>[4x]GPLGSSKTKPFTLPILTISEMSNSRFPVPIDSLHTSPTENIVVQCQNGRVTLDGELMGTTQLLPSQICAFRGTLTRSTSRASDQADTPTPRLFNYYWHIQLDNLNGTPYDPAEDIPAPLGTPDFRGKVFGVASQRNPDSTTRAHEAKVDTTSGRFTPKLGSLEITTESDDFDPNQPTKFTPVGVGVDNEAEFQQWSLPNYSGQFTHNMNLAPAVAPNFPGEQLLFFRSQLPSSGGRSNGVLDCLVPQEWVQHFYQESAPAQTQVALVRYVNPDTGRVLFEAKLHKLGFMTIAKNGDSPITVPPNGYFRFESWVNPFYTLAPMGTGNG

NoVs recognize specific glycan ligands as host attachment factors or receptors for infection. NoVs interact with HBGAs or other glycans through their capsid protrusions that are built by the dimeric protruding (P) domain of NoV capsid protein (VP1). Genogroup II (GII) noroviruses consist of human noroviruses (huNoVs) that generally bind histo-blood group antigens (HBGAs) as host factors and three porcine norovirus (porNoV) genotypes (GII.11/18/19) that form a genetic lineage lacking HBGA-binding ability. In this study, we solved the P protein crystal structures of a GII.11 porNoV (VA34) that was isolated from pig caecum contents in 1997 in Japan and a close-related GII.3 huNoV (TV24) that was isolated in 1977 in the USA, representing one of the earliest huNoV isolates, focusing on their HBSs compared with the previously known ones.

To this end, five oligosaccharides, including A type 1 trisaccharide, A tetrasaccharide (referred as A-tetra, Santa Cruz Biotechnology sc-285031), B trisaccharide (Sigma-B1422), H disaccharide (Sigma-F7012), and H type 2 trisaccharide (Sigma-F7297, see Materials and methods for their sequences) were co-crystallized with the TV24 P protein. However, only the electron density map of the A-tetra, the only tested tetrasaccharide, was found clearly on the TV24 P protein that was solved to 2.5 Å resolution (Figure 3(D and E)). The crystal structure of the TV24 P dimer-A-tetra complex was solved by Molecular Replacement (MR) and showed a clear electron density map (mFo-DFc) of the extra density of A-tetra at 2σ contour level. All four saccharide rings are modelled clearly, indicating the HBS at the conventional location like those of other GII NoVs, on the outmost surface of the viral capsid (Figure 3(D and E)). Besides, R452 forms Van der Waals interaction with the methyl group at position 6 of the Fuc ring. While this Fuc-binding site appears to be highly conserved among most GII NoVs, we noted that, unlike R452 in TV24 HBS, most other GII huNoV HBSs show an aromatic residue (Y, H or F) at this position forming Van der Waals interaction with the Fuc via their aromatic ring. A strong H bond with K363 (about 2.54 Å), and four water-bridged ones with A359, H360, E361, and S449 were found, making K363 particularly important for the A-tetra binding, but this appears not the case in other GII huNoV HBSs. Particularly, Glc forms two direct H bonds to R452 and another one with a water molecule, stabilizing the TV24-A-tetra complex.>MAHHHHHHMNRIDLEGRVVVITGGARGIGYAVAQRALRSGAAVALWDLDAERLARSERELAELGKVCAVTVDQTKEAQIEAAVGKTLAAFGAIDVLINCAGITGGNGTTWELEPDVWRQVIDVNLIGPYLVCRA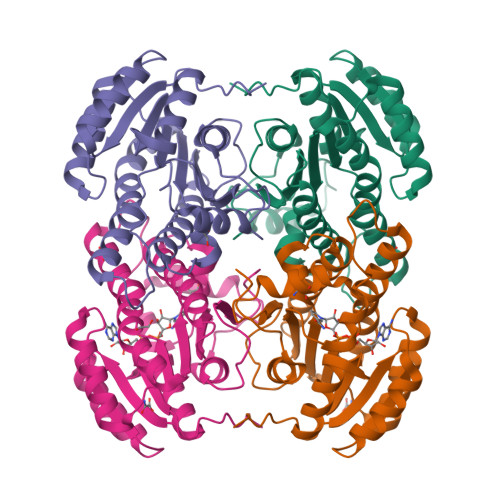VVPQMLKQGYGRIVNIASVAGKEGNPNASHYSASKAGLIGLTKSLGKELATKNILVNAVTPAAAKTEIFDSMKQEHIDYMLSKIPMNRFLLPDEAASLILWLGSEDCAFSTGSVFDLSGGRATY[2x]>KPKLHITMFPWVAIGHITPFIHLANELAKRGHSISILIPKKAHTQLGHNNLYPDLIKFHIVTVPHVEGLPAGAETASDIDITAKNPLAIAFDAMYEQVETLLYGLKPDIVFYDFADWIPKLAAQIGFKTVCYNVICASCMAIGIVPARHIPKDRPLTEEELMTPPEGYPSSTVVLRGQEARTLSFIGMDYGATKFDVRITAAMQGCDAIGIRTCRELEGPMCDYLSAQYNKPVFLSGPVLPESPKGPLEEKWEKWLNKFEPKSVVYCAFGSQMILQKNQFQELVLGFEMTGLPFFVALSKPHGADSIEEALPEGFLERVGDRGVVHGGWVQQTQILNHQSVGCFVSHCGFGSMWESLLSDSQIVLVPRLADQILNTRLLAEELKVAVEVERGDMGWFSKEDLCKAIKSVMDEESEVGKLVKKNHAKWRE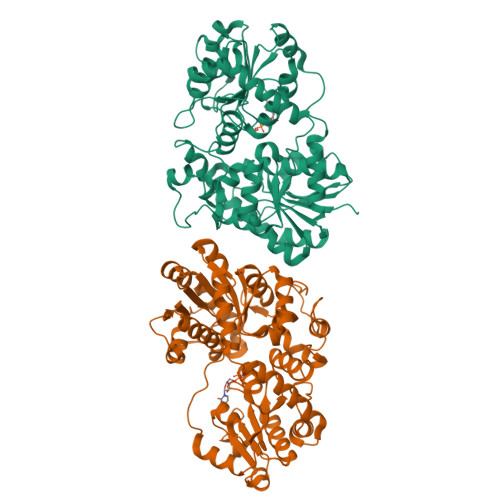TLVSPGYMDNYLEDFIQQLYG[2x]> MKSSHHHHHHENLYFQSNAESYTLTPEVGELIEKVRKAHQETFPALCQLGKYTTNNSSEQRVSLDIDLWDKFSELSTKCIIKTVEFAKQLPGFTTLTIADQITLLKAACLDILILRICTRYTPEQDTMTFSDGLTLNRTQMHHAGFGPLTDLVFAFANQLLPLEMDDAETGLLSAICLICGDRQDLEQPDRVDMLQEPLLEALKVYVRKRRP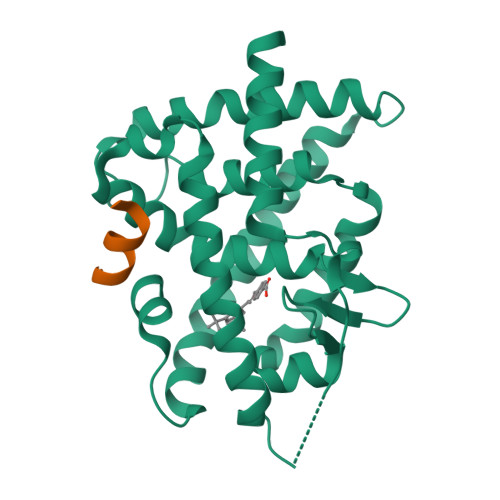SRPHMFPKMLMKITDLRSISAKGAERVITLKMEIPGSMPPLIQEMLENSEGLD;> RHKILHRLLQEGS> SFQASPSQSLYREIHQLISFKDVLPDKNLLPDWSSNKNPCTFDGVTCRDDKVTSIDLSSKPLNVGFSAVSSSLLSLTGLESLFLSNSHINGSVSGFKCSASLTSLDLSRNSLSGPVTTLTSLGSCSGLKFLNVSSNTLDFPGKVSGGLKLNSLEVLDLSANSISGANVVGWVLSDGCGELKHLAISGNKISGDVDVSRCVNLEFLDVSSNNFSTGIPFLGDCSALQHLDISGNKLSGDFSRAISTCTELKLLNISSNQFVGPIPPLPLKSLQYLSLAENKFTGEIPDFLSGACDTLTGLDLSGNHFYGAVPPFFGSCSLLESLALSSNNFSGELPMDTLLKMRGLKVLDLSFNEFSGELPESLTNLSASLLTLDLSSNNFSGPILPNLCQNPKNTLQELYLQNNGFTGKIPPTLSNCSELVSLHLSFNYLSGTIPSSLGSLSKLRDLKLWLNMLEGEIPQELMYVKTLETLILDFNDLTGEIPSGLSNCTNLNWISLSNNRLTGEIPKWIGRLENLAILKLSNNSFSGNIPAELGDCRSLIWLDLNTNLFNGTIPAAMFKQSGKIAANFIAGKRYVYIKNDGMKKECHGAGN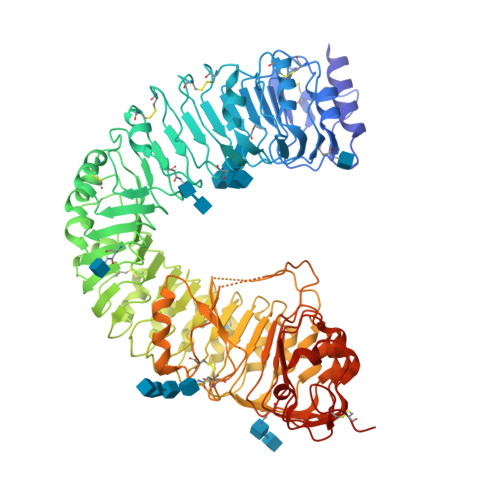LLEFQGIRSEQLNRLSTRNPCNITSRVYGGHTSPTFDNNGSMMFLDMSYNMLSGYIPKEIGSMPYLFILNLGHNDISGSIPDEVGDLRGLNILDLSSNKLDGRIPQAMSALTMLTEIDLSNNNLSGPIPEMGQFETFPPAKFLNNPGLCGYPLPRCDPSNADGYAHHQRSHHHHHH>APADNAADARPVDVSVSIFINKIYGVNTLEQTYKVDGYIVAQWTGKPRKTPGDKPLIVENTQIERWINNGLWVPALEFINVVGSPDTGNKRLMLFPDGRVIYNARFLGSFSNDMDFRLFPFDRQQFVLELEPFSYNNQQLRFSDIQVYTENIDNEEIDEWWIRGKASTHISDIRYDHLSSVQPNQN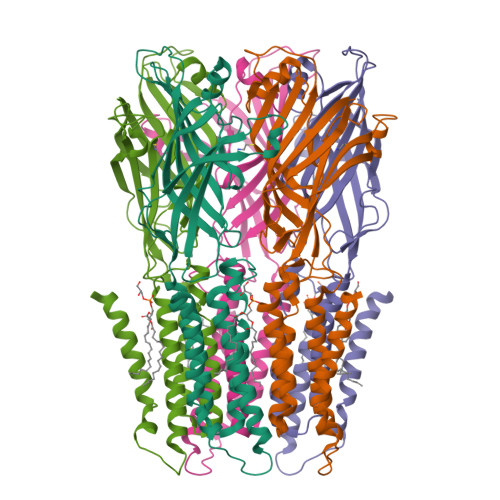EFSRITVRIDAVRNPSYYLWSFILPLGLIIAASWSVFWLESFSERLQTSFTLMLTVVAYAFYTSNILGRLPYTTYIDQMIIAGYGSIFAAILLIIFAHHRQANGVEDDLLIQRSRLAFPLGFLAIGCVLVIRFFTL[5x]> KVQ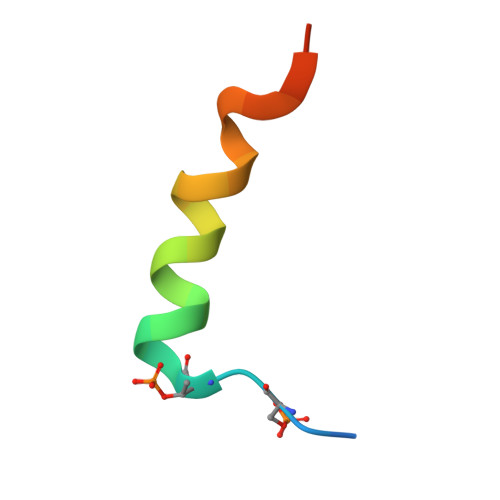PSPTVHTKEALGFIMNMFQAPTS Anion exchanger 2 (AE2) is an electroneutral Na+-independent Cl-/HCO3- exchanger belongs to the SLC4 transporter family. The widely expressed AE2 participates in a variety of physiological processes, including transepithelial acid-base secretion and osteoclastogenesis. Both the transmembrane domains (TMDs) and the N-terminal cytoplasmic domain (NTD) are involved in regulation of AE2 activity. Here, we report a 3.2 Å cryo-EM structure of the AE2 TMDs in complex with PIP2 and a 3.3 Å full-length mutant AE2 structure in the resting state without PIP2.

To investigate whether PIP2 regulates AE2 substrate exchange activity by allosterically disrupting the interface of the AE2 TMD and NTD, we introduced mutations (i.e., R932A, K1147A, and H1148A) into AE2 and then determined their structures. The mutant AE2 proteins were expressed and purified under the same conditions as wild-type AE2 and a map was reconstructed at an overall resolution of 3.3 Å. Analyses showed a strong density of the AE2 NTD which was not identified in the AE2IF/PIP2 state. The mutant AE2 TMD also adopted an inward-facing conformation with a RMSD of 1.704 Å compared with the TMD of AE2IF/PIP2 state. Because the substrate exchange activity of AE2 harboring the R932A/K1147A/H1148A mutations was significantly reduced, we designate this structure as the AE2IF/REST state. Aligning the TMD of the AE2IF/REST state with that of the AE2IF/PIP2 state by gate domain showed that inward rotational displacement of the AE2IF/REST core domain is greater (with a RMSD of 2.280 Å) than the displacement of core domain in the AE2IF/PIP2 state. PIP2 densities were absent from the dimer interface of the AE2IF/REST gate domain. Without the binding of PIP2, the intracellular half of TM7 shifted 6.2 Å (distance between Cα of I935) toward the core domain and the loop connecting TM6 to TM7 moved upward away from PIP2. Loops and β-sheets between TM10 and TM11 of AE2IF/REST state (missing in the AE2IF/PIP2 state due to their flexibility) stabilized the interface between the NTD and the TMD through several electrostatic interactions (between E508 and K1073, K348, and D1079) and hydrophobic interactions (between I347, F349, P363, L506, I510, P511, A1074, V1075, A1076 and P1077). Electrostatic interactions formed between E356 in the NTD, and K1157 and R1211 on the other protomer further stabilized the interaction between the AE2IF/REST TMD and NTD.

>[2x]MSSAPRRPAKGADSFCTPEPESLGPGTPGFPEQEEDELHRTLGVERFEEILQEAGSRGGEEPGRSYGEEDFEYHRQSSHHIHHPLSTHLPPDARRRKTPQGPGRKPRRRPGASPTGETPTIEEGEEDEDEASEAEGARALTQPSPVSTPSSVQFFLQEDDSADRKAERTSPSSPAPLPHQEATPRASKGAQAGTQVEEAEAEAVAVASGTAGGDDGGASGRPLPKAQPGHRSYNLQERRRIGSMTGAEQALLPRVPTDEIEAQTLATADLDLMKSHRFEDVPGVRRHLVRKNAKGSTQSGREGREPGPTPRARPRAPHKPHEVFVELNELLLDKNQEPQWRETARWIKFEEDVEEETERWGKPHVASLSFRSLLELRRTLAHGAVLLDLDQQTLPGVAHQVVEQMVISDQIKAEDRANVLRALLLKHSHPSDEKDFSFPRNISAGSLGSLLGHHHGQGAESDPHVTEPLMGGVPETRLEVERERELPPPAPPAGITRSKSKHELKLLEKIPENAEATVVLVGCVEFLSRPTMAFVRLREAVELDAVLEVPVPVRFLFLLLGPSSANMDYHEIGRSISTLMSDKQFHEAAYLADEREDLLTAINAFLDCSVVLPPSEVQGEELLRSVAHFQRQMLKKREEQGRLLPTGAGLEPKSAQDKALLQMVEAAGAAEDDPLRRTGRPFGGLIRDVRRRYPHYLSDFRDALDPQCLAAVIFIYFAALSPAITFGGLLGEKTQDLIGVSELIMSTALQGVVFCLLGAQPLLVIGFSGPLLVFEEAFFSFCSSNHLEYLVGRVWIGFWLVFLALLMVALEGSFLVRFVSRFTQEIFAFLISLIFIYETFYKLVKIFQEHPLHGCSASNSSEVDGGENMTWAGARPTLGPGNRSLAGQSGQGKPRGQPNTALLSLVLMAGTFFIAFFLRKFKNSRFFPGRIARVIGDFGVPIAILIMVLVDYSIEDTYTQKLSVPSGFSVTAPEKRGWVINPLGEKSPFPVWMMVASLLPAILVFILIFMETQITTLIISKKERMLQKGSGFHLDLLLIVAMGGICALFGLPWLAAATVRSVTHANALTVMSKAVAPGDKPKIQEVKEQRVTGLLVALLVGLSIVIGDLLRQIPLAVLFGIFLYMGVTSLNGIQFYERLHLLLMPPAAHPDVTYVKKVRTLRMHLFTALQLLCLALLWAVMSTAASLAFPFILILTVPLRMVVLTRIFTDREMKCLDANEAEPVFDEREGVDEYNEMPMPV>[4x]GPHMAAAAMAAAAGGGAGAARSLSRFRGCLAGALLGDCVGSFYEAHDTVDLTSVLRHVQSLEPDPGTPGSERTEALYYTDDTAMARALVQSLLAKEAFDEVDMAHRFAQEYKKD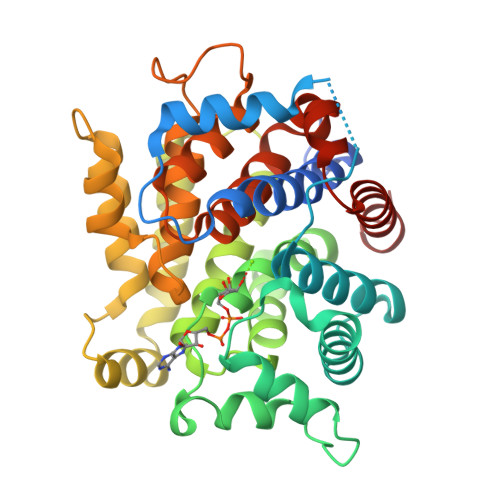PDRGYGAGVVTVFKKLLNPKCRDVFEPARAQFNGKGSYGNGGAMRVAGISLAYSSVQDVQKFARLSAQLTHASSLGYNGAILQALAVHLALQGESSSEHFLKQLLGHMEDLEGDAQSVLDARELGMEERPYSSRLKKIGELLDQASVTREEVVSELGNGIAAFESVPTAIYCFLRCMEPDPEIPSAFNSLQRTLIYSISLGGETDTIATMAGAIAGAYYGMDQVPESWQQSCEGYEETDILAQSLHRVFQKS>MEVGMIPRVYLGHEWFGAERILSEYQVPEDCGAQVLFLGIPRNAPEDGGNIEALEYEAYPEMAIKEMEKIRQETIEKFGVKEVFIHHRLGLVKIGEPSFLVLAVGGHREETFKACRYAVDETKKRVPIWKKEIFKEGKGEWVLGEKKNAS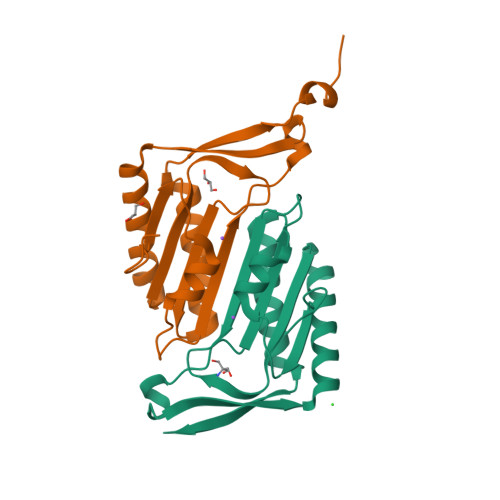GQTK[2x]> GSHMASMTGGQQMGRGSEFMRNELEEMQRRADQLADESLESTRRMLQLVEESKDAGIRTLVMLD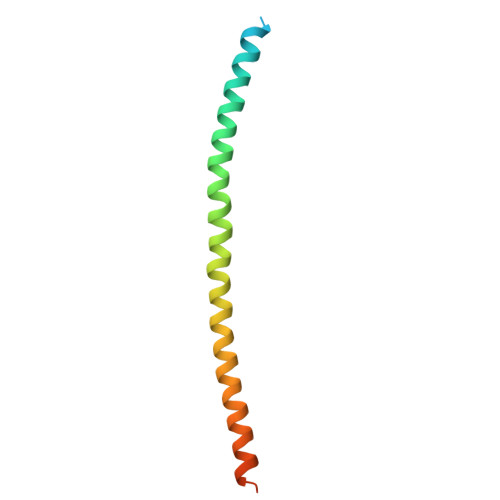EQGEQLDRVEEGMNHINQDMKEAEKNLKDLG> ALFDRLGRVVRANLNDLVSKAEDPEKVLEQAVIDMQEDLVQLRQAVARTIAEEKRTEQRLNQDTQEAKKWEDRAKLALTNGEENLAREALARKKSLTDTAAAYQTQLAQQRTMSENLRRNLAALEAKISEAKTKKNMLQARAKAAKANAELQQTLGGLGTSSATSAFERMENKVLDMEATSQAAGELAGFGIENQFAQLEASSGVEDELAALKAS

A prominent member of the PspA family is the vesicle-inducing protein in plastids 1 (Vipp1), also known as IM30 (inner membrane-associated protein of 30 kDa). Vesicle-inducing protein in plastids 1 (Vipp1) is critical for thylakoid membrane biogenesis and maintenance. Vipp1 appears to have two functions: in membrane maintenance (that is, during heat or light stress) and in thylakoid membrane (TM) biogenesis and/or remodeling. Vipp1 binds to negatively charged membranes and membrane binding depends on stored curvature elastic stress.

Using single-particle-based helical reconstruction, we resolved the structures of type I tubes at 5.1-Å resolution and two structures of type II tubes at 7.0-Å and 7.1-Å resolution. The type I and II tubes differ in their diameter and the arrangement of the monomers relative to the tube axis, as well as the diameter and thickness of the engulfed lipid bilayer tube. In contrast to the Vipp1 rings, the monomer orientation of the α1−α3 hairpin with respect to the tube axis is the same over the whole length of the tubes. Nevertheless, the monomer orientation among the tubes differs; in type I tubes, the α1−α3 hairpins are oriented parallel to the tube axis, while, in type II tubes, the hairpins are tilted approximately 45° relative to the tube axis. Remarkably, from rings over type II tubes to type I tubes, the α1−α3 hairpins accommodate a wide range of orientations along the tubulated membrane axis from perpendicular to parallel (from 90° to 0°) while essentially maintaining the same intermolecular contacts to stabilize the assembly. The here-determined structures of Vipp1 polymers in the presence of membranes indicated that helix α0 is immersed in the outer lipid leaflet of the bilayer. However, in contrast to SynPspA helix α0 that protrudes toward the bilayer, Vipp1 α0 lies flat in the membrane plane and appears to be partially submerged into the outer bilayer leaflet. The bilayer thickness in all three Vipp1 tubes remained nearly identical at 35 Å, although the inner leaflet radius changed with the tube diameter. Nevertheless, the same or similar intermolecular interactions of α0 with another α0 and α1 + α4, as observed previously in Vipp1 rings, are present in type I and II tubes.> MDKKKLLYWVGGGLVLILIWLWFRNRPAAQVASNWEGPPYMTYNQPQA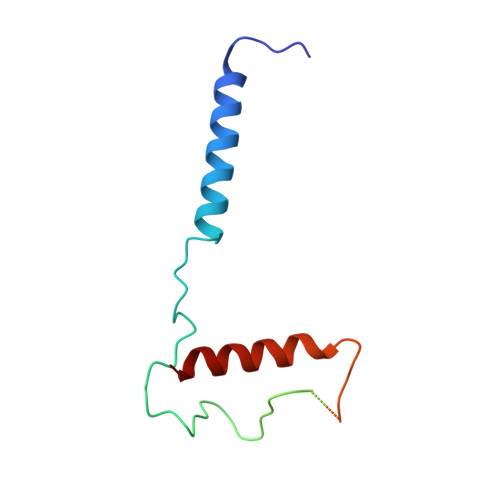GSVTLPVAGYTSPSPTLPNRNRSCGCNPAVSAAMAQGADLASKLTDSITSQLNDYASSLNDYLASQAGV(2S,3S)-3-{3-[2-chloro-4-(methylsulfonyl)phenyl]-1,2,4-oxadiazol-5-yl}-1-cyclopentylidene-4-cyclopropyl-1-fluorobutan-2-amine 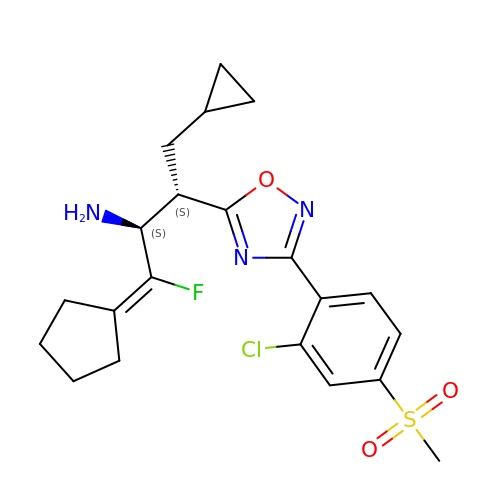| C21 H25 Cl F N3 O3 S | XCCSSVMRGIQMGF-LPHOPBHVSA-N>MGSSHHHHHHSSGMNRHTDTHYPSLADKVVLISGGASGIGRAFVEAFVAQGSRVAFLDLDAEAGQGLAHALGANSLFLPCDVRDIERLKACVAEVERTWGAVDVLINNAARDDRHALADVSVE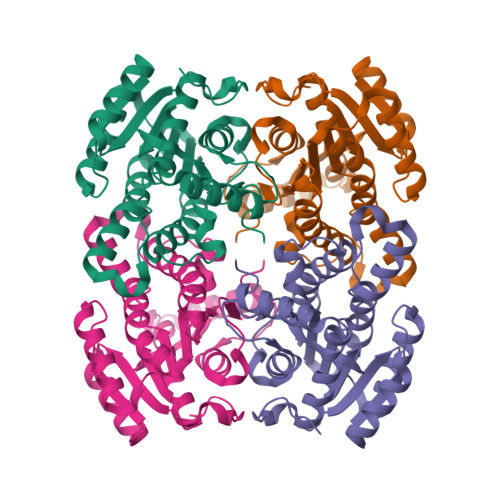YWDERMQTNLRHAFFAAQAVAPGMARRGSGAIINMGSISWMRGRPGMVCYTTAKAALNGMTRTLARELGGQGIRINSLVPGAIRTERQDAMWAADPAGLEAASQAFIDQQMLKFRLDASDCARLALFLASDDSRGCTGQNFVVDAGLSIQ[2x]> SMIFNVLTIFPQMFPGPLGVSNLGSALKKGLWTLNVFDIRAFANNKHNTVDDTPYGGGPGMLLRADVLGRCIDEVLSLHPNTKLMFTSPRGVSFTQDIARQTMNFDNI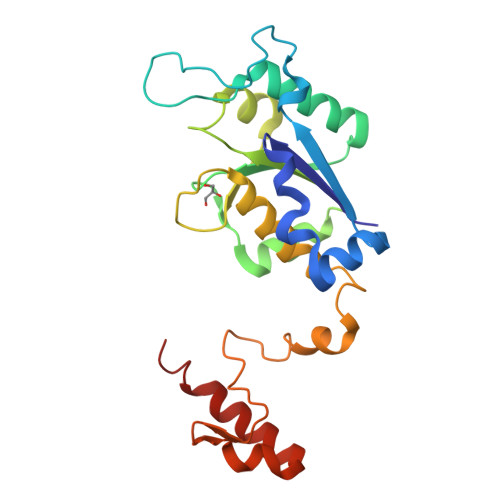TLLCGRFEGIDERVVDFYKLQEVSIGDYVLSGGELAAMVIIDTCVRMVPGVIGNAESLKQESMEGSLEYPQYTRPASWKGMEVPEVLLTGNHGEIEKWRRNASLSITAAR> ESPMSSDKGRNRWSRYIGSIHTMGFATRPTVKPVPIGSRLGFKKSVPKDLPLGKSLQHQHCSHLVRLIDTSQDRELGRMPEDVARILYPLLDYSEQVSLEPYLLINNGKRFSVGDNIYIRIDCYLTSQAFVRIEGGSILNKSFINDHGMDTRQLHRAGAIMALFDAINIQPVYGDTKNEMIPNYQENTVSSSQFQDEALNINQLKSFYRITQSAASLQNLPETTPDESLFKLQLRRYQKQSLSWMLKREYEYSHLSEKAAEVSIDGNSMNPLWKKFRWPSNSKQGTPNHEDDCFFYANLYTGEFSIEKPVIKTIINGGILADEMGLGKTISALALICTASYDEAHEKKIESTKKPSMKEMSSQVDSSPLRHSQHKHDTYAYRTTLIVVPMSLLNQWQSEFEKANKDLKKRCEIYYGNNIKDLRAYVLGPNAPSVIITTYGIIQSEYGRTSTSGLFNVVFFRIILDEGHTIRNRSTRTSKAVIALRSSRKWILTGTPIINRLDDLFSLVQFLNLEPWSHINYWKRYVSVPFEKGNYAQAFDVINAVLEPVLLRRTKNMKDVDGKPLVSLPPKEVIVEKLQLSSSEKRVYQSMLEDAENSVKEGLAKGDLLKNYTNILVHILRLRQVCCHLDLLKKTPDLGDPDLEDLENSTQNISSILMPKNIKSPKSSISQDKLDALSANFRDIHSASEQLPSFECAICTTECIEPLSAVSITECLHTFCEPCLAEYIEFQQNKKLSINCPYCRMPISEANVLKLKEPIDAERGYELISFHSHFQSTKIKALLRHLKQIQETSPGEQIIVFSQFSSFLDILEIELRSHLPRDQVIIYKFDGRLDMKERTRILEQFHDKDLSCIKLLLLSLKTGGVGLNLTCASRAFMMDPWWSPGMEDQAIDRIHRIGQQQTVKVVRFIIDNSVEEKMLRIQERKRMLGDIVEGDEAERRQKRIEEIQMLFQ

Rad5 possesses a ubiquitin ligase activity and catalyzes the Lys63-linked ubiquitin-chain modification of the proliferating cell nuclear antigen (PCNA). Rad5 also possesses ATP hydrolysis-driven DNA translocase activity, through which it catalyzes the regression of replication forks. The remaining part of ScRad5 contains three distinct domains, including a HIP116 and Rad5 N-terminal (HIRAN) domain, a superfamily 2 (SF2) DNA translocase motor domain of the Snf2 sub-family (Snf2 domain), and a ubiquitin ligase RING domain embedded in the Snf2 domain. These distinct domains endow Rad5 with DNA damage site recognition, replication fork remodeling, and ubiquitin ligase activities.

We screened through a number of fungal species and were able to purify a nearly full-length fragment of Rad5 from the yeast K. lactis (KlRad5, containing residues 163–1114) and crystallize it in the absence of DNA. Structures of the mercury-derivatized and native crystals were refined to resolutions of 3.3 Å and 3.6 Å, respectively. Minimal differences were observed between these structures. One native crystal was used for diffraction data collection, data from three mercury-derivatized crystals were merged and presented. The structure revealed an elongated shape of KlRad5 spanning 140 Å in the longest dimension. The HIRAN, Snf2, and RING domains are well resolved in the structure. The HIRAN domain and the two lobes in the Snf2 domain are nearly aligned in a line, the RING domain is located on the side. In contrast, the RING domain has little contact with either the Snf2 or the HIRAN domain. In our structure, motifs I/II have located over 20 Å away from motif VI, suggesting that KlRad5 rests in an ATPase-inactive state in the absence of DNA.>[2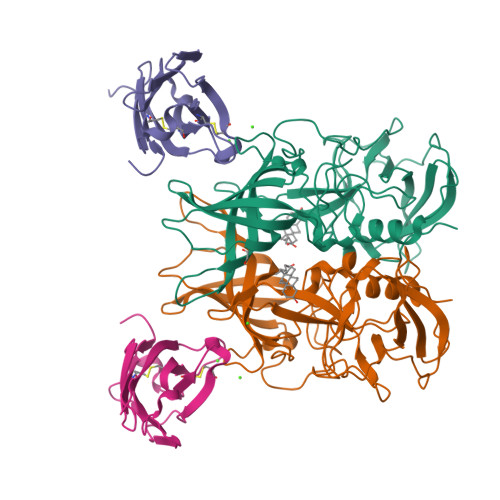x]MVDLPVIQPRLCTHARWPAPVYGLLVDPSLPSNPQWQNGRVHVDGTLLGTTPISGSWVSCFAAEAAYKFQSGTGEVATFTLIEQDGSAYVPGDRAAPLGYPDFSGQLEIEVQTETTKTGDKLKVTTFEMILGPTTNADQAPYQGRVFASVTAAASLDLVDGRVRAVPRSIYGFQDTIPEYNDGLLVPLAPPIGPFLPGEVLLRFRTYMRQIDTADAAAEAIDCALPQEFVSWFASNAFTVQSEALLLRYRNTLTGQLLFECKLYNEGYIALSYSGSGPLTFPTDGIFEVVSWVPRLYQLASVGS;>[2x]MEDPVTGPEEVSGQEQGSLTVQCRYTSGWKDYKKYWCQGVPQRSCKTLVETDASEQLVKKNRVSIRDNQRDFIFTVTMEDLRMSDAGIYWCGITKGGLDPMFKVTVNIGPVPT(3S,6S)-3,6-bis(4-hydroxybenzyl)piperazin-2-one 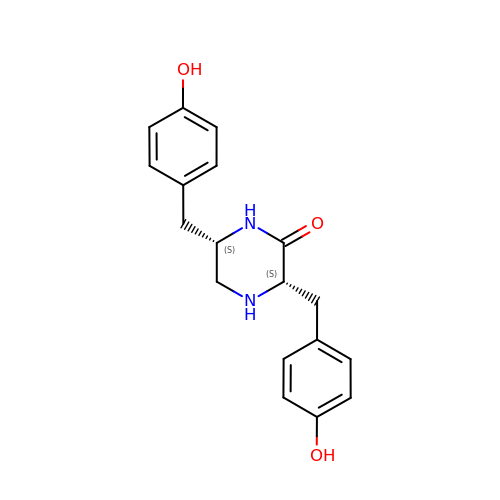| C18 H20 N2 O3 | WZUSPDRVLVOBKD-YOEHRIQHSA-N(2R)-1-methoxypropan-2-amine | C4 H11 N O | 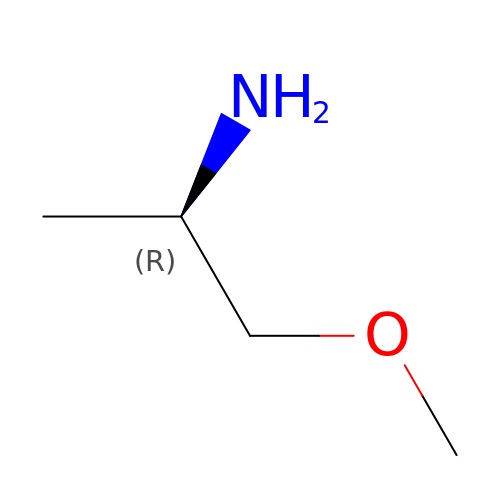NXMXETCTWNXSFG-SCSAIBSYSA-N> QLWRCQRQFLQHQRLRACQRFIHRRAQF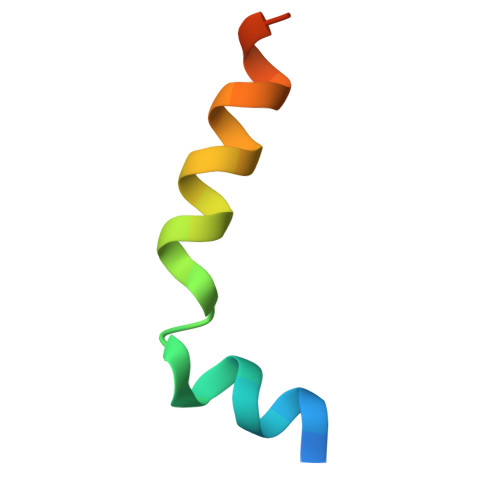GGQPD> YPPEVSISGYDNNWYLGQNEATLTCDARSNPEPTGYNWSTTMGPLPPFAVAQGAQL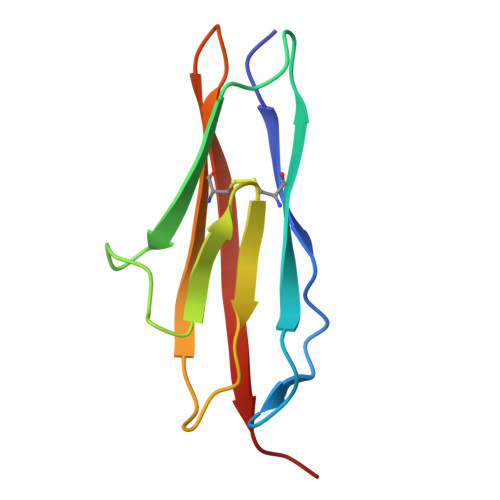LIRPVDKPINTTLICNVTNALGARQAELTVQVKEGP> STLHISDLILQASPVVQLVMLILLLASIFSWYLIAKLHMSYKKARQDDEHFQKMFWSGAELNTLYNNAQLNSKRSGLEDIFYQGLSE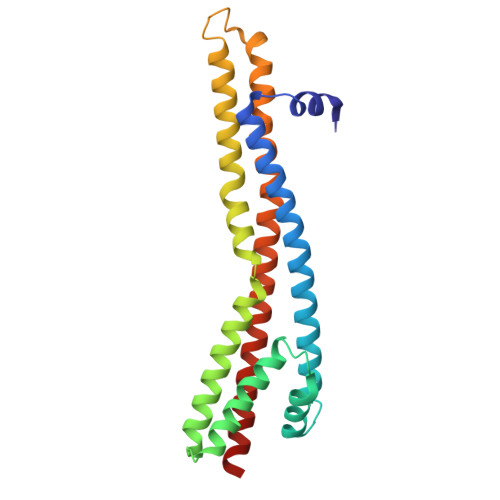FFKLKKRQAPTSQMIEGTERILRVGLSRDQGSLEYGLGTLASIGSVAPYIGLFGTVWGIMNAFIGLAAVDQVTLATVAPGIAEALIATAIGLFAAIPAVLAFNHFTAKSESVYSDRALFAEEMIALLQRQSVG>M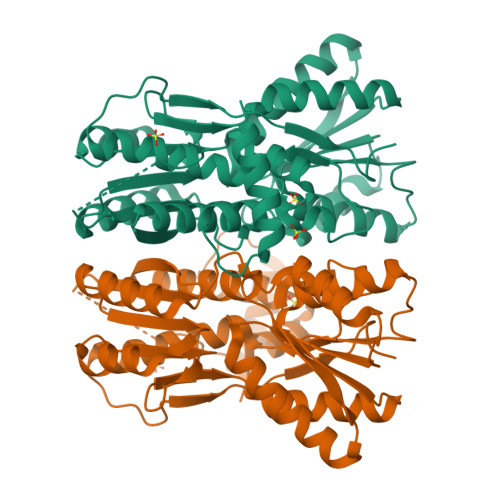TVTIYDVAREARVSMATVSRVVNGNQNVKAETKNKVNEVIKRLNYRPNAVARGLASKKTTTVGVIIPDISNIYYSQLARGLEDIATMYKYHSIISNSDNDPEKEKEIFNNLLSKQVDGIIFLGGTITEEMKELINQSSVPVVVSGTNGKDAHIASVNIDFTEAAKEITGELIEKGAKSFALVGGEHSKKAQEDVLEGLTEVLNKNGLQLGDTLNCSGAESYKEGVKAFAKMKGNLPDAILCISDEEAIGIMHSAMDAGIKVPEELQIISFNNTRLVEMVRPQLSSVIQPLYDIGAVGMRLLTKYMNDEKIEEPNVVLPHRIEYRGTTK[3x]> NYMGNPWTEYMAKYDIEEVHGSGIRVDLGEDAEVAGTQYRLPSGKCPVFGKGIIIENSNTTFLKPVATGNQDLKDGGFAFPPTNPLISPMTLNGMRDFYKNNEYVKNLDELTLCSRHAGNMNPDNDKNSNYKYPAVYDYNDKKCHILYIAAQENNGPRYCNKDQSKRNSMFC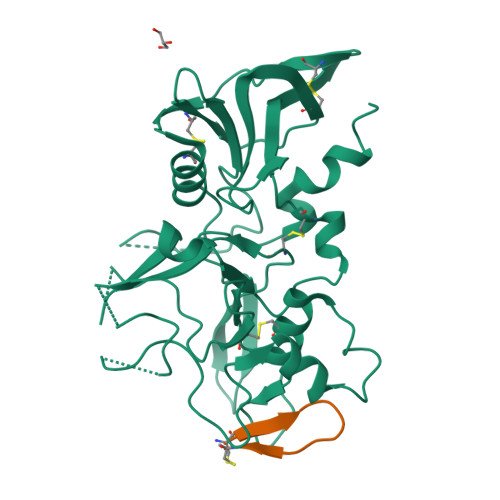FRPAKDKLFENYTYLSKNVVDNWEEVCPRKNLENAKFGLWVDGNCEDIPHVNEFSANDLFECNKLVFELSASDQPKQYEQHLTDYEKIKEGFKNKNASMIKSAFLPTGAFKADRYKSHGKGYNWGNYNRETQKCEIFNVKPTCLINNSSYIATTALSHPIEVE;> CFTARMSPPQQIC> ASMTGGQQMGRGSSLTACPEESPLLVGPMLIEFNIPVDLKLVEQQNPKVKLGGRYTPMDCISPHKVAIIIPFRNRQEHLKYWLYYLHPILQRQQLDYGIYVINQAGESMFNRAKLLNVGFKEALKDYDYNCFVFSDVDLIPMNDHNTYRCFSQPRHISVAMDKFGFSLPYVQ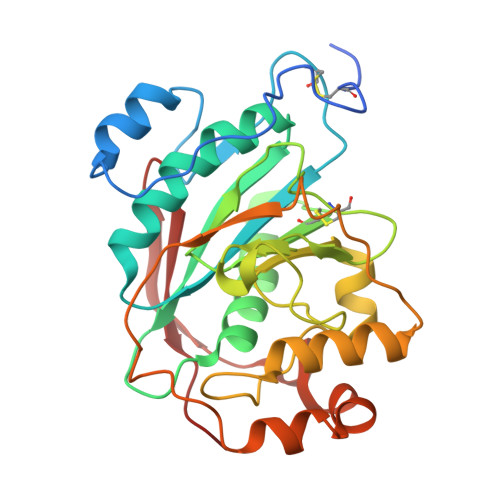YFGGVSALSKQQFLSINGFPNNYWGWGGEDDDIYNRLAFRGMSVSRPNAVIGKTRMIRHSRDKKNEPNPQRFDRIAHTKETMLSDGLNSLTYMVLEVQRYPLYTKITVDIGTPS>[2x]LKCNKLIPIAYKTCPEGKNLCYKMMLASKKMVPVKRGCINVCPKNSALV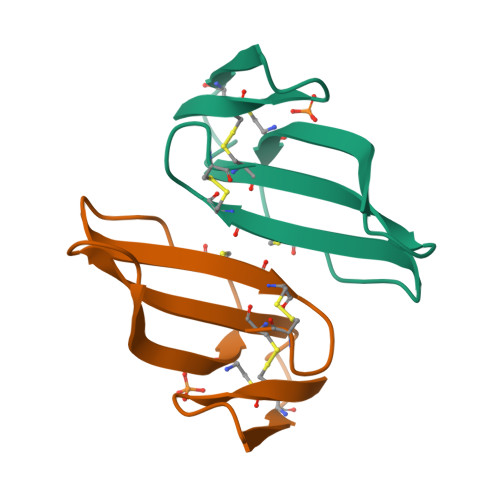KYVCCSTDRCN>MKVLFLTANEFEDVELIYPYHRLKEEGHAVYIASFERGTITGKHGYSVKVDLTFDKVNPAEFDALVLPGGRAPERVRLNAKAVSIARKMFSEGKPVASICHGPQILISAGVLRGRKGTSYPGIKDDMINAGVEWVDAEVVVDGNWVS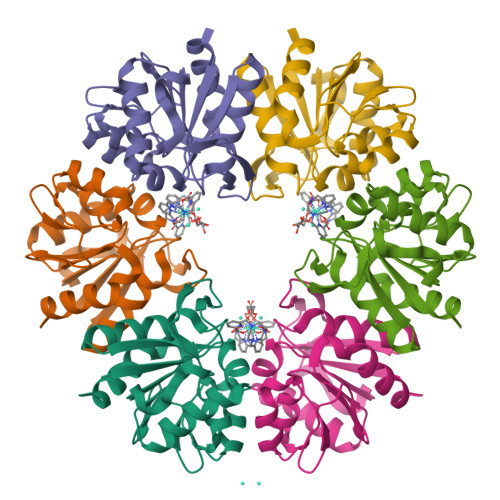SRVPADLYAWMREFVKLLK[3x]> MATATVATTPEGIPVIILKEGSSRTYGKEALRANIAAVKAIEEALKSTYGPRGMDKMLVDSLGDITITNDGATILDKMDLQHPTGKLLVQIAKGQDEETADGTKTAVILAGELAKKAEDLLYKEIHPTIIVSGYKKAEEIALKTIQEIAQPVTINDTDVLRKVALTSLGSKAVAGAREYLADLVVKAVAQVAELRGDKWYVDLDNVQIVKKHGGSVNDTQLVYGIVVDKEVVHPGMPKRIENAKIALLDASLEVEKPELDAEIRINDPTQMHKFLEEEENILKEKVDKIAATGANVVICQKGIDEVAQHYLAKKGILAVRRAKKSDLEKLARATGGRVISNIDELTSQDLGYAALVEERKVGEDKMVFVEGAKNPKSVSILIRGGLERVVDETERALRDALGTVADVIRDGRAVAGGGAVEIEIAKRLRKYAPQVGGKEQLAIEAYANAIEGLIMILAENAGL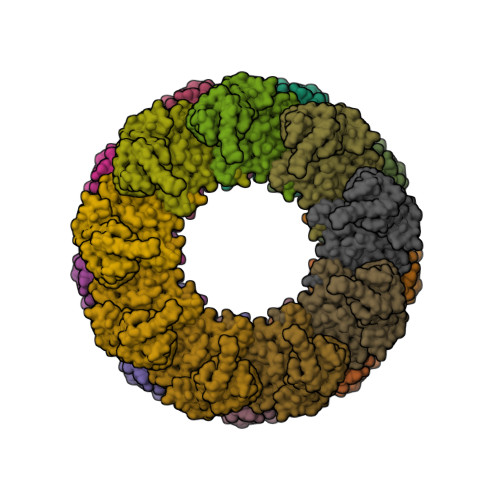DPIDKLMQLRSLHENETNKWYGLNLFTGNPEDMWKLGVIEPALVKMNAVKAATEAVTLVLRIDDIVAAGKKSGSEPSGKKEKDKEEKSSED> VEVDCSRFPNTTNEEGKDVLVCTEDLRPICGTDGVTHSECLLCAYNIEYGTNISKEHDGECREAVPMDCSRYPNTTSEEGKVMILCNKALNPVCGTDGVTYDNECVLCAHNLEQGTSV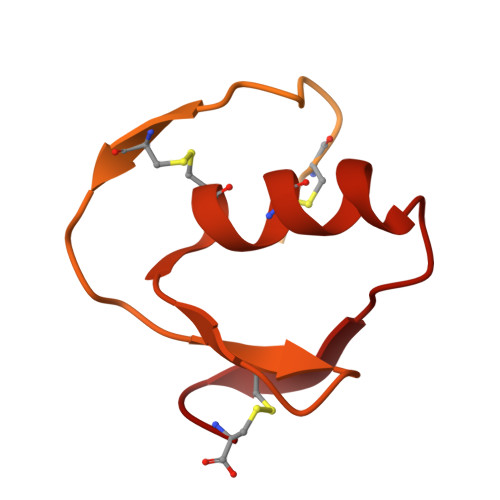GKKHDGECRKELAAVSVDCSEYPKPACTLEYRPLCGSDNKTYGNKCNFCNAVVESNGTLTLSHFGKC Hence, allelic variation in genes for the translation factor eIF4E has accounted for differential susceptibility of their hosts to Pepper mottle virus (PepMoV), Pepper vein mottle virus (PMMV), Potato virus Y (PVY), Tobacco etch virus (TEV), Lettuce mosaic virus (LMV), Barley mild mosaic virus (BaMMV), Barley yellow mosaic virus (BaYMV), Bean yellow mosaic virus (BYMV), Zucchini yellow mosaic virus (ZYMV;) and Pea seed-borne mosaic virus (PSbMV). Resistance-breaking isolates of these viruses are not uncommon and comparative genetic and molecular analyses have identified the virus-genome linked protein (VPg) as the predominant avirulence factor. This is supported by in vitro biochemical and yeast two-hybrid assays that point to a direct interaction between VPg and the product of the dominant eIF4E susceptibility allele (eIF4ES), which does not occur with the resistance variant, eIF4ER. In this paper we describe this structure and report the impact of a series of point mutations in and around the cap-binding pocket of pea eIF4E on infection with PSbMV, and use the protein crystal structure to provide a three-dimensional framework for interpreting these data. The monomer is comprised of a central 8-stranded anti-parallel β-sheet flanked by α-helices, although one face of the β-sheet is largely undecorated by α-helices and this is where the cap-binding site resides.

In preparation for a structure-function analysis of pea eIF4E in relation to PSbMV susceptibility we determined the crystal structure of pea eIF4EΔN51 by molecular replacement, using the wheat orthologue as a template. We therefore designed a version of the pea protein truncated at the position equivalent to that used for the crystallization of the wheat protein. The pea protein was co-crystallised with the cap analogue m7GTP. The X-ray data revealed eight independent copies of eIF4E in the crystallographic asymmetric unit, which assemble as two distorted tetramers, and within each tetramer a maximum of approximately 600 Å2 of protein surface is buried between pairs of subunits. Since only monomers were detected in solution, we conclude that these assemblies are simply crystal packing artefacts. The cap-binding pocket of eIF4E structures are characterised by a pair of tryptophan residues (W75 and W121 in the pea protein), which form π-stacking arrangements with the 7-methyl-guanine moiety (m7G) of the cap. These residues are located on the β1–β2 and β3–β4 loops, respectively, defining, in our views, the left and right hand sides of the pocket. The m7GTP ligand is further stabilised in the cap-binding site by a van der Waals contact with W180 on β5, and additional polar interactions with E122 on the β3–β4 loop, R171 on β5, and K176 on β6. A superposition of the wheat structure with chain H of the pea structure gives a root mean square deviation of 0.708 Å over 171 structurally equivalent residues.

>[8x]MPHLLENSWTFWFDTPAAKSKQAAWGSSMRPIYTFSTVEEFWSIYNNIHHPGKLAVGADFYCFKHKIEPKWEDPICANGGKWTANYPKGKSDTSWLYTLLAMIGEQFDHGDEICGAVVNVRGRAEKISIWTKNASNEAAQVSIGKQWKEFLDYNETMGFIFHDDARKLDRNAKNKYVV> MGNPMNTTQLGKSLFQWQVEQEESKLANISQDQFLSKDADGDTFLHIAVAQGRRALSYVLARKMNALHMLDIKEHNGQSAFQVAVAANQHLIVQDLVNIGAQVNTTDCWGRTPLHVCAEKGHSQVLQAIQKGAVGSNQFVDLEATNYDGLTPLHCAVIAHNAVVHELQRNQQPHSPEVQELLLKNKSLVDTIKCLIQMGAAVEAKDRKSGRTALHLAAEEANLELIRLFLELPSCLSFVNAKA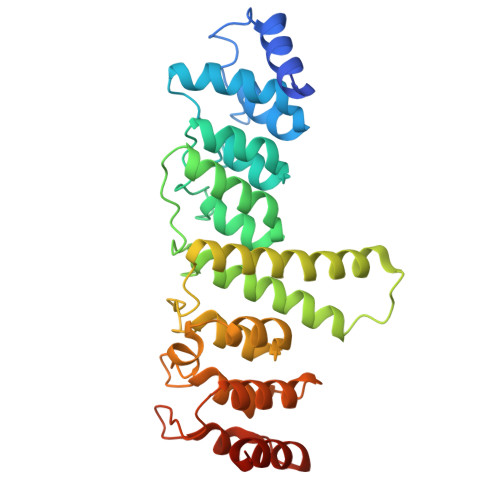YNGNTALHVAASLQYRLTQLDAVRLLMRKGADPSTRNLENEQPVHLVPDGPVGEQIRRILKGKSIQQRAPPY> MHHHHHHSSGRENLYFQGGDKPPPLCGAIPASGDYVARPGDKVAARVKAVDGDEQWILAEVVSYSHATNKYEVDDIDEEGKERHTLSRRRVIPLPQWKANPETDPEALFQKEQLVLALYPQTTCFYRA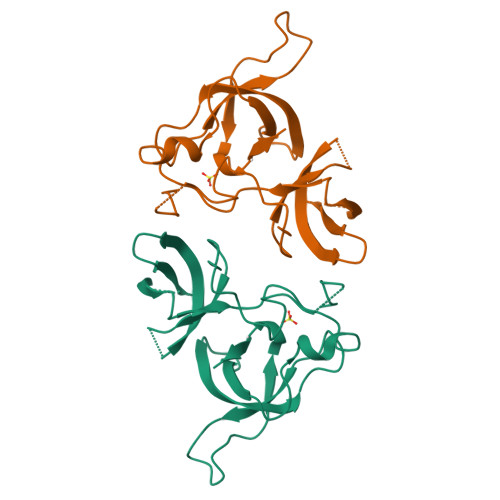LIHAPPQRPQDDYSVLFEDTSYADGYSPPLNVAQRYVVACKEPKKK>[2x]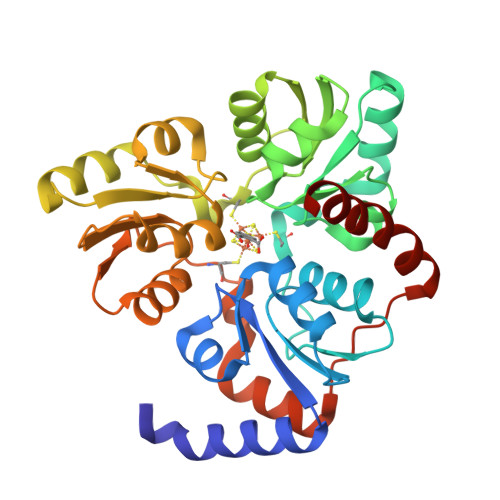HHHHHHMVDEILKLKKEKGYIILAHNFQIPELQDIADFVGDSLQLARKAMELSEKKILFLGVDFMAELVKILNPDKKVIVPDRSATCPMANRLTPEIIREYREKFPDAPVVLYVNSTSECKTLADVICTSANAVEVVKKLDSSVVIFGPDRNLGEYVAEKTGKKVITIPENGHCPVHQFNAESIDAVRKKYPDAKVIVHPECPKPVRDKADYVGSTGQMEKIPERDPSRIFVIGTEIGMIHKLKKKFPDREFVPLEMAVCVNMKKNTLENTLHALQTESFEVILPKEVIEKAKKPILRMFELMG>[10x]MHAYLHC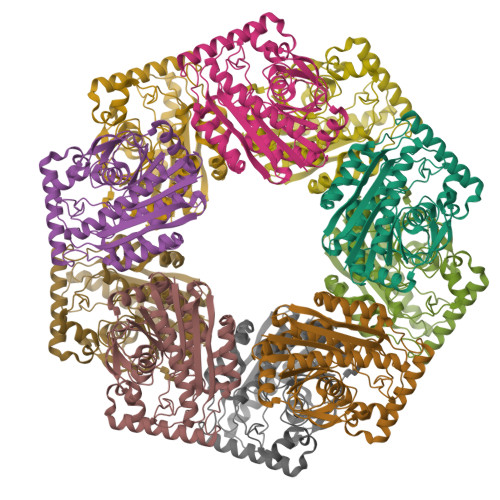LSHSPLVGYVDPAQEVLDEVNGVIASARERIAAFSPELVVLFAPDHYNGFFYDVMPPFCLGVGATAIGDFGSAAGELPVPVELAEACAHAVMKSGIDLAVSYCMQVDHGFAQPLEFLLGGLDKVPVLPVFINGVATPLPGFQRTRMLGEAIGRFTSTLNKRVLFLGSGGLSHQPPVPELAKADAHMRDRLLGSGKDLPASERELRQQRVISAAEKFVEDQRTLHPLNPIWDNQFMTLLEQGRIQELDAVSNEELSAIAGKSTHEIKTWVAAFAAISAFGNWRSEGRYYRPIPEWIAGFGSLSARTEN> SNNSVYTSFMKSHRCYDLIPTSS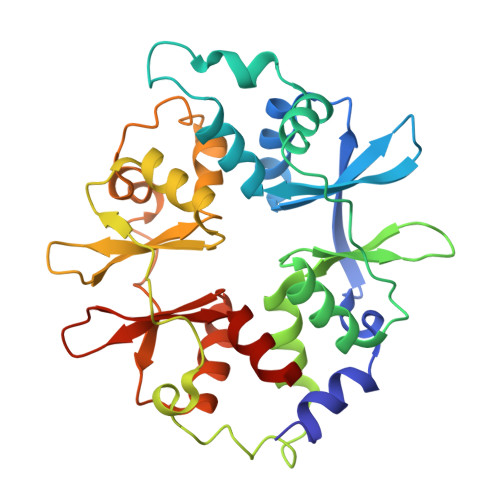KLVVFDTSLQVKKAFFALVTNGVRAAPLWDSKKQSFVGMLTITDFINILHRYYKSALVQIYELEEHKIETWREVYLQDSFKPLVCISPNASLFDAVSSLIRNKIHRLPVIDPESGNTLYILTHKRILKFLKLFITEFPKPEFMSKSLEELQIGTYANIAMVRTTTPVYVALGIFVQHRVSALPVVDEKGRVVDIYSKFDVINLAAEKTYNNLDVSVTKALQHRSHYFEGVLKCYLHETLETIINRLVEAEVHRLVVVDENDVVKGIVSLSDILQALVLTGG> MESLPVIAAPSMWTRPQIKDFKEKIQQDADSVITVGRGEVVTVRVPTHEEGSYLFWEFATDNYDIGFGVYFEWTDSPNTAVSVHVSESSDDDEEEEENIGCEEKAKKNANKP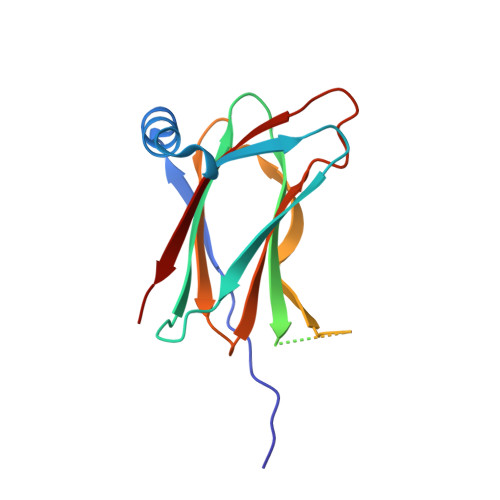LLDEIVPVYRRDCHEEVYAGSHQYPGRGVYLLKFDNSYSLWRSKSVYYRVYYTR>[4x]EVDPRLYFENRSKFIQDQKDKGINPYPHKFERTISIPEFIEKYKDLGNGEHLEDTILNITGRIMRVSASGQKLRFFDLVGDGEKIQVLANYSFHNHEKGNFAECYDKIRRGDIVGIVGFPGKSKKGELSIFPKETILLSACLHMLPMKYGLKDTEIRYRQRYLDLLINESSRHTFVTRTKIINFLRNFLNERGFFEVETPMMNLIAGGANARPFITHHNDLDLDLYLRIATELPLKMLIVGGIDKVYEIGKVFRNEGIDNTHNPEFTSCEFYWAYADYNDLIKWSEDFFSQLVYHLFGTYKISYNKDGPENQPIEIDFTPPYPKVSIVEEIEKVTNTILEQPFDSNETIEKMINIIKEHKIELPNPPTAAKLLDQLASHFIENKYNDKPFFIVEHPQIMSPLAKYHRTKPGLTERLEMFICGKEVLNAYTELNDPFKQKECFKLQQKDRE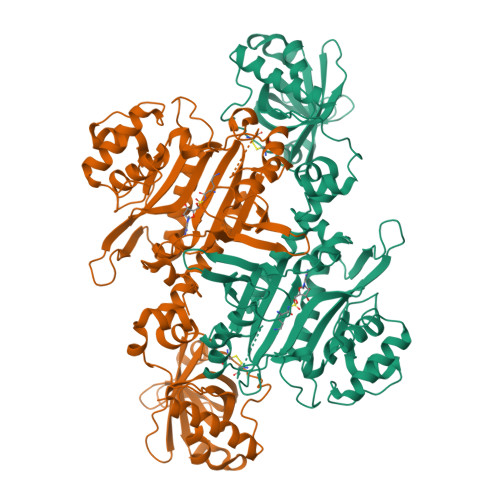KGDTEAAQLDSAFCTSLEYGLPPTGGLGLGIDRITMFLTNKNSIKDVILFPTMRPAN Parallel to this two other proteins have emerged – primarily from genetic studies – as being factors that significantly modulate plasma triglyceride levels and CAD. These proteins, human angiopoietin-like protein 3 (Angptl3; also known as Ang5) and angiopoietin-like protein 4 (Angptl4) are, as the names suggest, related structurally to angiopoietins which are involved in angiogenesis via their interaction with the Tie2 (tyrosine kinase with immunoglobulin and endothelial growth factor homology domain-2) receptor. Here we determined the structures of the fibrinogen-like domains of Angptl3 and Angptl4, structures which offer new insights into reported loss of function mutations, the mechanisms of action of the proteins and open up the possibility of rational design of low molecular weight inhibitors. The fibrinogen-like domains of Angptl3 and Angptl4 form compact structures and, according to fibrinogen nomenclature, can be divided to 3 subdomains A, B and P.

The Angptl4 crystal contains 1 molecule per asymmetric unit and the visible polypeptide chain begins with Leu184 and ends with Met400, hence 6 amino acids of the C-terminus are not visible. There is one break in the mainchain of Angptl4 at Gln370, suggesting the loop that it is in is flexible. The B subdomain of Angptl4 is similar to that of Angptl3; however, the extended β-sheet is formed by four antiparallel β-strands and instead of the long β-strand β6 in Angptl3, it contains 2 short β-strands (β6 and β7), which form an antiparallel β-hairpin and are connected via α-helix α5 and an extended solvent exposed loop. In contrast to Angptl3, the regular secondary structure of the P subdomain of Angptl4 is comprised of only three short α-helices (α6, α7 and α8). Similarly to Angptl3 it contains one disulfide bond (Cys341 and Cys354). Similarly angiopoietins 1 and 2 are the closest structural homologs of Angptl4, with rms deviation of 2.7 Å (200 equivalent Cα positions) and 2.6 Å (200 equivalent Cα positions) respectively. However, the β-sheet of the B subdomain is narrower in Angptl4 than that of homologous structures and β-strand β6 is much shorter and turns away from the β-sheet towards the solvent and together with β7, α5 and an extended loop creates a separate solvent exposed element in the structure. Analysis of the electrostatic surface potential of the fibrinogen-like domain of Angptl3 and Angptl4 revealed that the electrostatic charge is relatively evenly distributed over the majority of the surface of both molecules, except for the presence of an extended positively charged patch at the bottom of the P subdomain of Angptl4, the surface that is most likely involved in the functional interactions. For Angptl4 there are two reported mutations (P251T and R371Q) which are linked to increased triglyceride levels. Of the six mutants made in Angptl4, three gave no soluble protein (G223R, W349C and G361S) while one resulted in greatly reduced protein yields (R384W).

> MHHHHHHMLPRDCQELFQVGERQSGLFEIQPQGSPPFLVNCKMTSDGGWTVIQRRHDGSVDFNRPWEAYKAGFGDPHGEFWLGLEKVHSITGDRNSRLAVQLRDWDGNAELLQFSVHLGGEDTAYSLQLTAPVAGQLGATTVPPSGLSVPFSTWDQDHDLRRDKNCAKSLSGGWWFGTCSHSNLNGQYFRSIPQQRQKLKKGIFWKTWRGRYYPLQATTMLIQPMAAEAAS> E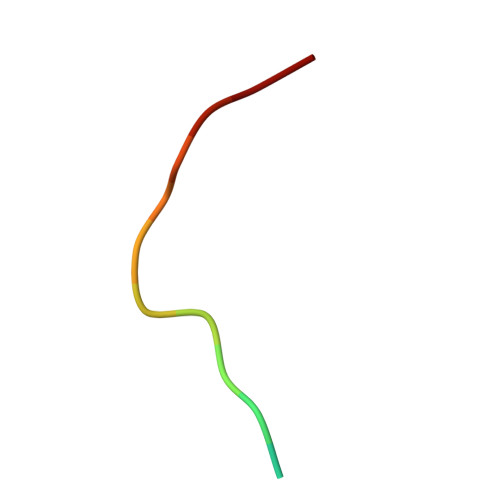GNPYVPVHFDASV The aryl hydrocarbon receptor (AHR), a member of the basic helix–loop–helix (bHLH) Per–Arnt–Sim (PAS) family of transcription factors, plays important roles in regulating xenobiotic metabolism, cellular differentiation, stem cell maintenance, as well as immunity. From the N- to C-terminus, AHR comprises a basic helix-loop-helix (bHLH) domain for DNA binding, two tandemly arranged PAS domains (termed PAS-A and PAS-B) for dimerization, and a transcription activation domain12. The ligand binding site of AHR has been mapped to its PAS-B domain. Here, we present multiple crystal structures of the Drosophila AHR PAS-B domain, including its apo, ligand-bound, and AHR nuclear translocator (ARNT) PAS-B-bound forms.

Only the PAS-B domain of Drosophila AHR (dAHR) is soluble. We then performed crystallographic studies on purified dAHR PAS-B. Diffraction-qualified crystals were successfully obtained, and the structure was determined at a resolution of 2.6 Å. Topologically, dAHR PAS-B is arranged as βA-βB-αC-αD-αE-βF-βG-βH-βI-αJ and resembles a baseball catcher’s mitt, with the six β-strands forming the palm and three helices (αC, αD and αE) forming the opposing thumb. Next, we compared our dAHR PAS-B structure with the previously reported PAS-B structure of hypoxia-inducible factor-2α (HIF-2α), as the latter is also a bHLH-PAS protein capable of binding ARNT and whose activity can be modulated by synthesized molecules. Although the overall folding was similar, superimposing the two structures gave a root-mean-square deviation (rmsd) of 4.5 Å over 106 equivalent Cα atoms, which indicated comparable differences. The C-termini adopt opposite conformations in the two structures, with dAHR PAS-B folding into a helix (αJ), while HIF-2α presents as a loop. In addition, part of the residues between αE and αD folded into a short helix (αD’) in HIF-2α, while this helix was not observed in dAHR PAS-B. Other minor differences are observed within the αE, βH, αC and αD regions. These observations suggest that dAHR PAS-B has a similar overall fold while adopting some unique features compared to HIF-2α PAS-B. CASTp39 assigns 440 Å3 and 680 Å3 cavity volumes for dAHR PAS-B and mAHR PAS-B, respectively. Combined with the fact that the activation of dAHR is constitutive and ligand-independent, we infer that dAHR PAS-B might be in an intrinsically active conformation.

> GSIPHKENMFKSKHKLDFSLVSMDQRGKHILGYADAELVNMGGYDLVHYDDLAYVASAHQELLKTGASGMIAYRYQKKDGEWQWLQTSSRLVYKNSKPDFVICTHRQLMDEEGHDLLGKR> QFAKPEDAVKYRQSAVTLMASHFGRMTPVVKGQAPYDAAQIKANVEVLKTLSALPWAAFGPGTEGGDARPEIWSDAASFKQKQQAFQDNIVKLSAAADAGDLDKLRAAFGDVGASCKACHDAYRKK

Cytochromes c′ occur in methanotrophic, denitrifying and photosynthetic bacteria and have proposed roles in protection against nitrosative stress, NO trafficking during denitrification or pathogen defence. All cytochromes c′ have a 4 α-helix bundle structure containing a heme centre with a solvent exposed proximal His ligand and a buried hydrophobic distal pocket with a non-coordinated residue (Leu or Phe, rarely Met or Tyr) in a position to exert steric influence on the binding of diatomic gases. Unusually, cytochromes c′ are able to utilize both heme faces (distal and proximal) as a means of discriminating NO from other diatomic gases. In order to understand the factors controlling distal versus proximal NO coordination, we have examined NO binding to AXCP variants in which the occluding distal residue Leu16 is replaced with residues that are smaller (Ala, Val), of comparable size (Ile) or larger (Phe).

All of the tertiary structures are similar to wt AXCP and only salient points concerning the heme region are discussed here. Ferrous structures show the different residues at position 16 to lie over the heme in a similar manner to that of Leu16 in wt AXCP (Fig. S4†) with the exception of L16A where the side chain is essentially truncated.>MSAKILCVLYDDPVDGYPKTYARDDLPKIDHYPGGQTLPTPKAIDFTPGALLGSVSGELGLRKYLEANGHTFVVTSDKDGPDSVFERELVDADVVISQPFWPAYLTPERIAKAKNLKLALTAGIGSDHVDLQSAIDRGITVAEVTYCNSISVAEHVVMMILGLVRNYIPSHDWARKGGWNIADCVEHSYDLEGMTVGSVAAGRIGLAVLRRLAPFDVKLHYTDRHRLPEAVEKELGLVWHDTREDMYPHCDVVTLNVPLHPETEHMINDETLKLFKRGAYIVNTARGKLADRDAIVRAIESGQLAGYAGDVWFPQPAPKDHPWRTMKWEGMTPHISGTSLSAQARYAAGTREILECFFEGRPIRDEYLIVQGGALAGTGAHSYSKGNATG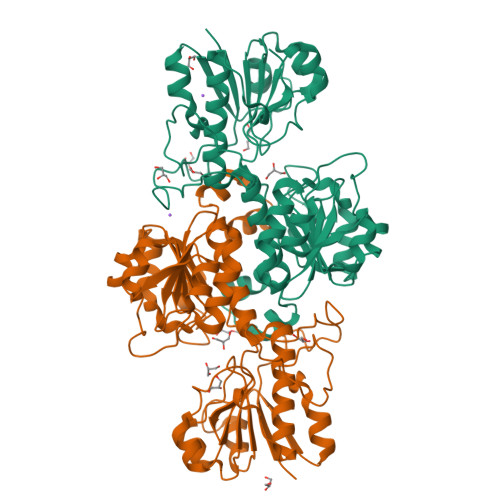GSEEAAKFKKAGALEVLFQGPHHHHHHHHHH[4x]> MARIKDNNAPKRFNKISIGLASPESILAESRGEVLKPETINYRTHKPERDGLFCERIFGPVKDYECACGKYKRIRYRGIVCDRCGVEVTEKKVRRDRVGHINLVVPVAHIWYFRSLPNKIGYLLGLPSKKLDMIIYYERYVVIQPGIAKGPEGEEIHKLDFLTEEEYLNILESLPSENQYLEENDPNKFIAKMGAECLIDLLARIDLEQLSYELRHKANTETSKQRKTEALKRLQVVEALRESQDNRENNPEWMIMKVIPVIPPELRPLVPLDGGRFATSDLNDLYRRVIIRNNRLKRLMEIKAPEVILRNEKRMLQEAVDSLFDNTRKASAVKTESNRPLKSLSDSLKGKQGRFRQNLLGKRVDYSARSVIVVGPEMKLYECGLPKDMAAELYKPFIIRKLIERGIVKTVKSAKKIIDKKEPVVWDILENVLKGHPVLLNRAPTLHRLGIQAFQPKLIEGKAIRLHPLACTAFNADFDGDQMAVHLPLGPEAILEAQLLMLASQNILNPANGSPITVPSQDMVLGLYYMTKEKRSTPEEPVIGEGLTFYSSEEVEIAFNERKVALNAIIKVRTKDFNEAGELVNKIIETTVGRVLFNTVVPEQAGYINTVLNKKSLRNIIGDILAVTDVPTTADFLDKIKTMGYEFAFKGGLSFSLGDIIIPKEKHEMIAEANEQVDGIMMNYNMGLITFNERYNQVIDVWTSTNAMLTELAMKRIREDKQGFNSVYMMLDSGARGSKEQIRQLTGMRGLMAKPKKSTAGGGEIIENPILSNFKEGLSILEYFISTHGARKGLADTALKTADAGYLTRRLVDVSQDVIINTEDCGTLRGIEVEALKKNEEVVETLGERILGRVSLHDVYNPLTEELILKAGQEISEADVKKVEAAPIEKVEVRSPLTCEAAQGICAKCYGRNLATNKMVQRGEAVGVVAAQSIGEPGTQLTLRTFHVGGIAGNISEDSKLEAKFDGIAEIEDLRVVEGVDNGGGKSDIVISRTSEIKIVDAKTGITLSTNNIPYGSQLFVKNGEKITKGTVICQWDPYNGVIVSEFTGQIAYENIEQGMTYQVEIDEQTGFQEKVISESRNKRLIPTLLIKDGKGETIRSYNLPVGSHLMVDNGEKIKEGKILVKIPRKSAKAGDITGGLPRVTELFEARNPSNPAVVTEIDGVVSFGKIKRGNREIIIESKAGEVK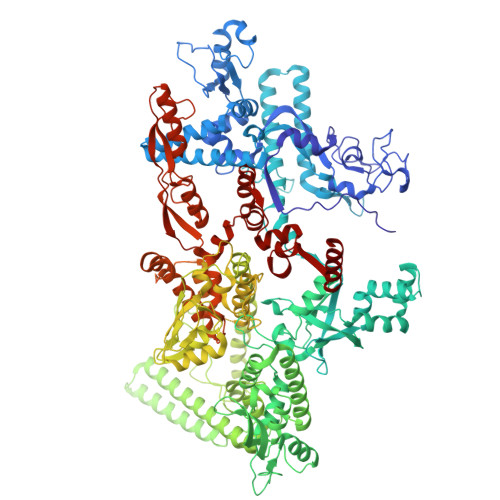KYLVKLSNQILVQENDYVRAGMALSDGSITPEDILAIKGPSAVQQYLVNEVQEVYRLQGVKINDKHFEVVVRQMMRKVQIQDSGDTTFLENQLVHKDDFINENDEIFGKKVVEDAGDSERLKPGQIVTARQLRDENSILRREDKTLVTARDAVAATATPILQGITRASLQTKSFISAASFQETTKVLNEAAVNGKVDTLEGLKENVIVGHKIPAGTGMRDYDSIIVGSKEEYDEIMARKEEFKF>[4x]ADQRRDFIDIESKFALRTPEDTAEDTCHLIPGVAESVATCHFNHSSKTFMVIHGWTVTGMYESWVPKLVAALYKREPDSNVIVVDWLSRAQEHYPVSAGYTKLVGQDVARFINWMEEEFNYPLDNVHLLGYSLGAHAAGIAGSLTNKKVNRITGLDPAGPNFEYAEAPSRLSPDDADFVDVLHTFTRGSPGRSIGIQKPVGHVDIYPNGGTFQPGCNIGEAIRVIAERGLGDVDQLVKCSHERSIHLFIDSLLNEENPSKAYRCSSKEAFEKGLCLSCRKNRCNNLGYEINKVRAKRSSKMYLKTRSQMPYKVFHYQVKIHFSGTESETHTNQAFEISLYGTVAESENIPFTLPEVSTNKTYSFLIYTEVDIGELLMLKLKWKSDSYFSWSDWWSSPGFAIQKIRVKAGETQKKVIFCSREKVSHLQKGKAPAVFVKCHDKSLNKKSG;>QTQQEE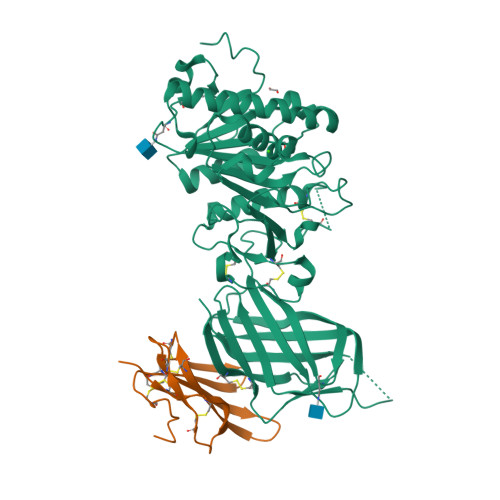EEEDEDHGPDDYDEEDEDEVEEEETNRLPGGRSRVLLRCYTCKSLPRDERCDLTQDCSHGQTCTTLIAHGNTESGLLTTHSTWCTDSCQPITKTVEGTQVTMTCCQSSLCNVPPWQSSRVQDPTG[4x]>[2x]SNAMSQFMNLEGKVALVTGASRGIGKAIAELLAERG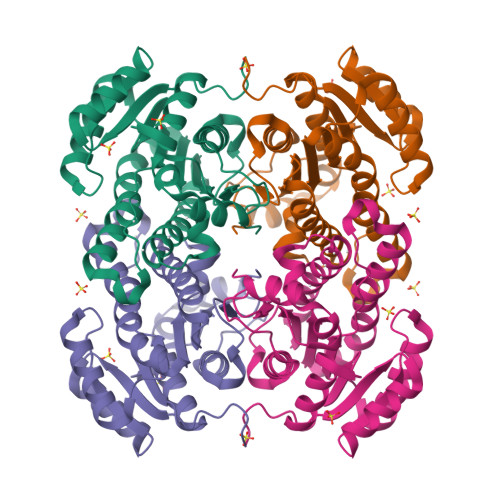AKVIGTATSESGAQAISDYLGDNGKGMALNVTNPESIEAVLKAITDEFGGVDILVNNAAITRDNLLMRMKEEEWSDIMETNLTSIFRLSKAVLRGMMKKRQGRIINVGSVVGTMGNAGQANYAAAKAGVIGFTKSMAREVASRGVTVNTVAPGFIETDMTKALNDEQRTATLAQVPAGRLGDPREIASAVAFLASPEAAYITGETLHVNGGMYMI>GTIYPRNPAMYSEEARLKSFQNWPDYAHLTPRELASAGLYYTGIGDQVQCFACGGKLKNWEPGDRAW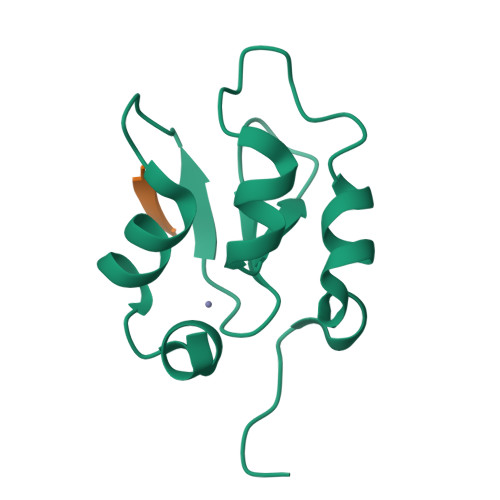SEHRRHFPNCFFVLGRNLN[2x];> AVPI> GPLGSMEKVNEERDAVFEDHIGDRRRSVRSLLEEAFADEMEKTSYDVEVADTPQPHIPIRFRHPPIAGPVHDVFGDAIHDIFQKMMKRGQAVDFCHWVSHLIATEIDEKFSEVAFRDVQYNPDIYVTDSTTEAKKLFNDKIWPAIDKILQQNAETCPILSEKWSGIHVSGDQLKGQRHKQEDRFLAYPNGQYMDRGEDPISVLAVFDGHGGHECSQYAAGHLWETWLEVRKSRDPSDSLEDQLRKSLELLDERMTVRS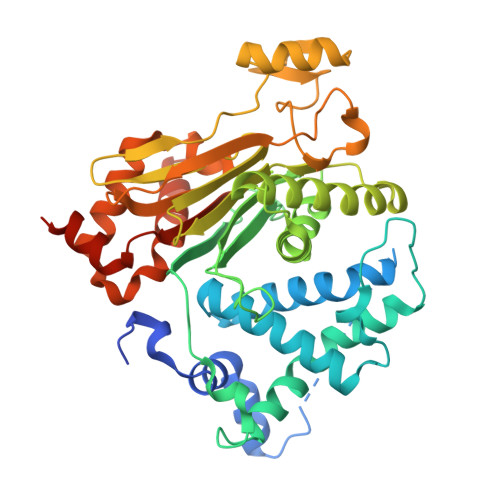VKECWKGGSTAVCCAIDMDQKLMALAWLGDSPGYVMSNIEFRQLTRGHSPSDEREARRVEEAGGQLFVIGGELRVNGVLNLTRALGDVPGRPMISNEPETCQVPIESSDYLVLLACDGISDVFNERDLYQLVEAFANDYPVEDYAELSRFICTKAIEAGSADNVSVVIGFLRPPQDVWKLMKHESDDEDSDVTDEE>PPRKVLIISAGASHSVALLSGDIVCSWGRGEDGQLGHGDAEDRPSPTQLSALDGHQIVSVTCGADHTVAYSQSGMEVYSWGWGDFGRLGHGNSSDLFTPLPIKALHGIRIKQIACGDSHCLAVTMEGEVQSWGRNQNGQLGLGDTEDSLVPQKIQAFEGIRIKMVAAGAEHTAAVTEDGDLYGWGWGRYGNLGLGDRTDRLVPERVTSTGGEKMSMVACGWRHTISVSYSGALYTYGWSKYGQLGHGDLEDHLIPHKLEALSNSFISQISGGWRHTMALTSDGKLYGWGWNKFGQVGVGNNLDQCSPVQVRFPDDQ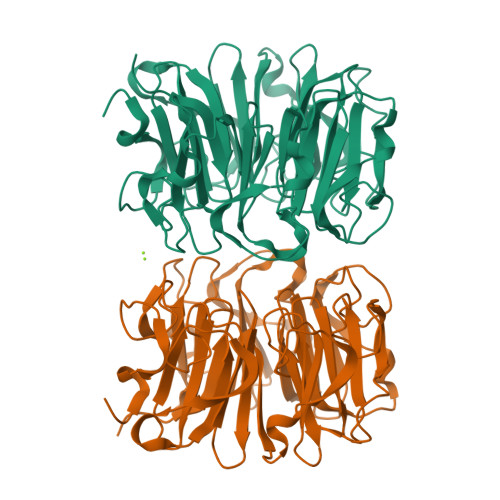KVVQVSCGWRHTLAVTERNNVFAWGRGTNGQLGIGESVDRNFPKIIEALSVDGLEHHHHHH[4x]> MATASHNIDDILQLKDDTGVITVTADNYPLLSRGVPGYFNILYITMRGTNSNGMSCQL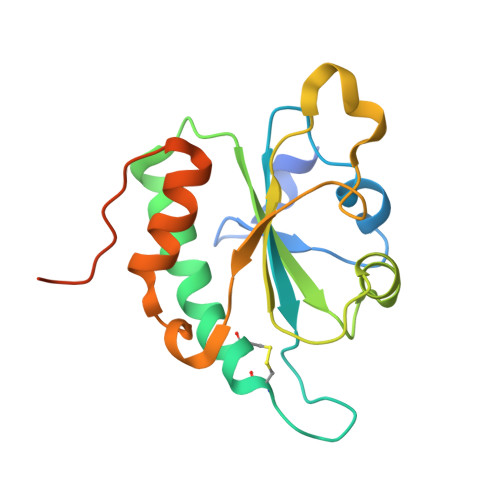CHDFEKTYHAVADVIRSQAPQSLNLFFTVDVNEVPQLVKDLKLQNVPHLVVYPPAESNKQSQFEWKTSPFYQYSLVPENAENTLQFGDFLAKILNISITVPQAFNVQEEFHHHHHHHHHH>MTDQGLEGSNPVDLSKHPSGIVPTLQNIVSTVNLDCKLDLKAIALQARNAEYNPKRFAAVIMRIR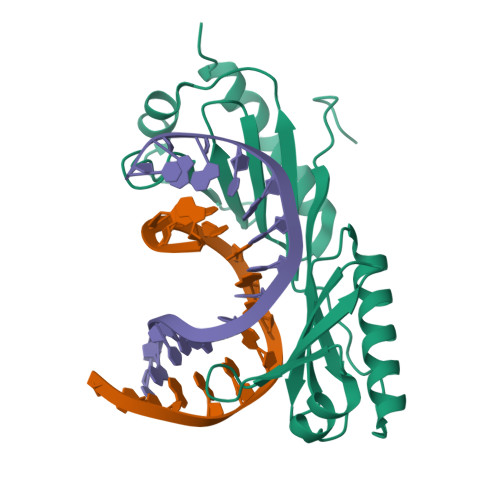EPKTTALIFASGKMVCTGAKSEDFSKMAARKYARIVQKLGFPAKFKDFKIQNIVGSCDVKFPIRLEGLAYSHAAFSSYEPELFPGLIYRMKVPKIVLLIFVSGKIVITGAKMRDETYKAFENIYPVLSEFRKIQQ[2x]>[2x]MTDSPFRAWDVFMVRTPVGYAYPTPLSNSGFDSPASSPGFGEGEFPPDAPVPSDVSGHGAGSSEASVRASGRPPAGDHLSLLRAACEDGPLMEAVELASPSLAGLLARVARGDTGGLKDKRLRRAALALLRYDIRMRTRPTPFGLFAGVSGGRFDTSAKWLAGTGHRTRTRADMEWLLSAVHRLERDRVLLAGVTVQAHQTLTVRGDRIVLDCPSALGKPLNGSTRSTVSARRSPVVAEILGAARRPVLAGRLAQSVAQRFELPADRVTGLLADMAAQELLITALRPPLDGDDPLQHVLDVVAAAEARAGSPAEAMSSESAALVAALREVDARCHAYDRTAVGQGRRELAELIQSTRRVHPHDTPLHVDLRIDLEVRLPEVVRTEIERAAEALWRLSPPRRGMRALRRYHEAFLERYGADRAVPLLELLDDTRGLGPPAGYKWPPSETPAGPQEEPRRSAALARLVAKAARRGEREIVIDEETIAELAYDEAAPADLPNSLELGVHVVAPSLDELSAGTFRVVLAPGPGSHHAGATLGRFTGLLPDVDAE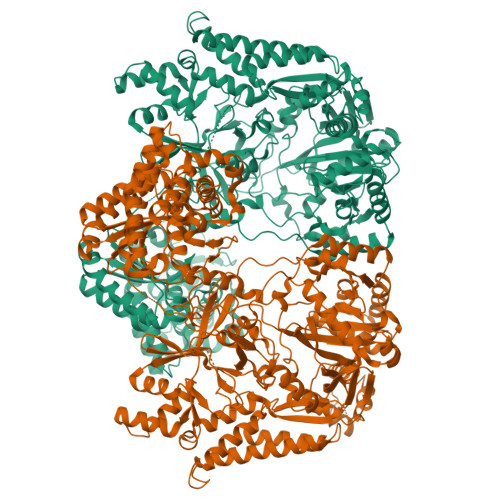SAARQAGRPLHIQDAVAADVAFIPRSGRAANLAHTPSYSGRRISVGLPDSGRAQEIPLDELGVGANLERLCLVHLPTGREVVPALPNMVSAFAQAPNPARLLFELGLEGQRLWEPWDWGALSEMPFLPGVRYGRTLLAAPLWRMDQLRGPADDSGPAADWDAALDRWRAEWNVPRRVLAVSMDQRLLLDLDDAWHRVLLRDELRRTPELIAQQVAGDEEGWLDRGDAGFPGHLAEIVVPLERRDRHAARPPHIRATVSGREPTGAGGPWLYLRLRVPRRNQDDFLRDQVPVLVRAGIEHGADRWFFIRYSDTAGQHLRVRFRGEREKLWAGLLPEIGARLVEWQRQGLLAGHELGQYDPEYERYGGDALAEFTETAFQHDSAAAISLLRLTRRAGFRYTLDEVTAISAAALADAFGPPAPVVEPVPLVGGLQWAPDLFDGDPAAAWMSSTGGRRELPPDYRRDPARWQKLIDPTGGWPLLRADEDGCQVLAALESRDEAVRRFGTAYREAFRPTDSPSTQLRLVGSLLHMTCNRLIGGSAERERSVLGLARGAVQDNLNRRRHLA> ADPVRSSSRTPSDKPVAHVVANPQAEGQLQWLNRRANALLANGVELRDNQLVVPSEGLYLIYSQVLFKGQGCPSTHVLLTHTISRIAVSYQTKVNLLSAIKSPCQRETPEGAEAKPWYEPIYLGGVFQLEKGDRLSAEINRPDYLDFAESGQVYFGIIALEFRS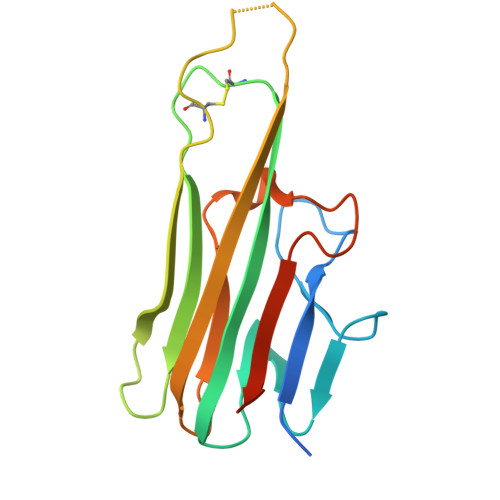GRLVPR> MSHHHHHHSMSKNILDM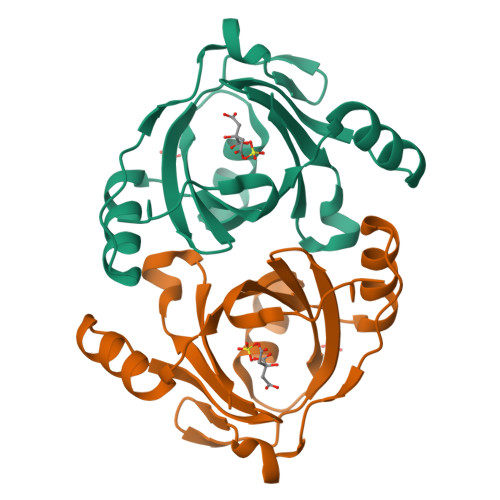RNTVQIGIVVRDIEESLQNYAEFFGVEKPQWFWTDDYSKAHTKFNGRPTKARAKLAFFELGPLQLELIEPDENPSTWREFLDKNGEGIHHIAFVVKDMDRKVEELYRKGMKVIQKGDFEGGRYAYIDTLRALKVMIELLENY>[3x]ALALDT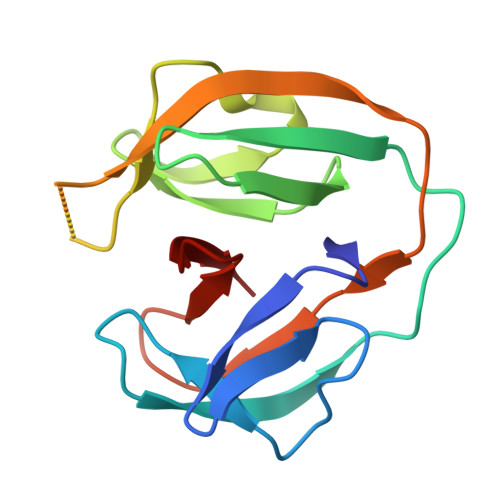PLPTPSGWTTMGDVAVGDHLLGPDGEPTRVVADTDVMLGRPCYVVEFSDGTAIVADAQHQWPTEHGVRITANLRAGMHTVVSASGGRGGTALLAPAVQITAVRRRPSVPVRCVEVDNPEHLYLAGPGMVPTHN>SNAMTKTIEVRNPRTGKFDYVIIPPPPRLLAQQCNRARRAQSRWQELGVEGRITTLQQWKQAILSRREQLTEALVNDTGRLSITVLEIDSFLASIDRWCGLAPELLQTSAKNTSIPFIALQQSLVPYPLVGVISPWNFPLTLSMIDTIPALLAGCAVVVKPSEIAPRFVAPLLMALNTVPELRDVLIFVEGGGETGANLINYVDFVCFTGSVATGREVAETAARRFIPAYLELGGKDPAIVLESANLELATSAILWGAVVNTGQSCLSIERIYVAESKFEEFYHQLIAKAHRLQLAYPLVEDGAIGPIIAEKQAGIINDHILDAVEKGAVIHCGGKVEELGGGWWCRPTVMTNVNHSMKVMTEETFGPIMPVMPFPDVEEAVYLANDTIYGLSAAVFAGSEDEALKVARQLNAGAISINDAALTAM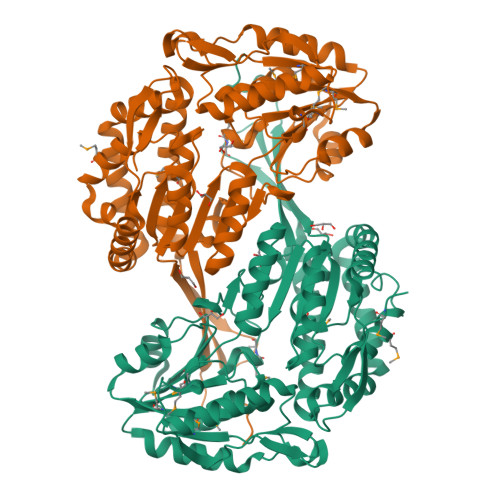MHEGEKNAFNFSGLGGSRVGAAGLKRFLRKQAFLIKTNSTSDPWWFDK[4x]>GAMDPEFAWEKQQRKTFTAWCNSHLRKAGTQIENIDEDFRDGLKLMLLLEVISGERLPKPERGKMRVHKINNVNKALDFIASKGVKLVSIGAEEIVDGNAKMTLGMIWTIILRFAIQDISVEETSAKEGLLLWCQRKTAPYKNVNVQNFHISWKDGLAFNALIHRHRPELIEY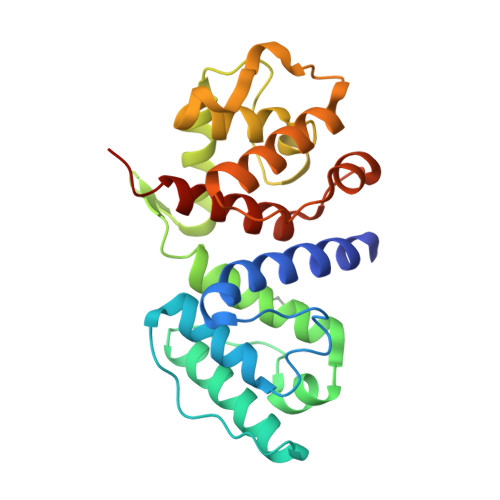DKLRKDDPVTNLNNAFEVAEKYLDIPKMLDAEDIVNTARPDEEAIMTYVSSFYHAFSGALDELN[2x]> QGSMGSKRQWALEDFEIGRPLGKGKFGNVYLAREKQSKFILALKVLFKAQLEKAGVEHQLRREVEIQSHLRHPNILRLYGYFHDATRVYLILEYAPLGTVYRELQKLSKFDEQRTATYITELANALSYCHSKRVIHRDIKPENLLLGSAGELKIADFGWSVHAPSSRRTTLCGTLDYLPPEMIEGRMHDEKVDLWSLGVLCYEFLVGKPPFEANTYQETYKRISRVEFTFPDFVTEGARDLISRLLKHNPSQRPMLREVLEHPWITANSSKPS

Aurora A is a serine/threonine protein kinase that plays an important role in controlling early stages of mitosis, including centrosome maturation and separation, mitotic entry, and bipolar spindle formation. Localization and enzymatic activity of Aurora A are regulated by its interaction with the spindle assembly factor TPX2. We have used fragment-based, structure-guided lead discovery to develop small molecule inhibitors of the Aurora A-TPX2 protein–protein interaction (PPI). The initial fragment hits identified from screening with the ATP site blocked by a high-affinity inhibitor were very weakly active, but guided by continuous crystallographic analysis of the inhibitors in complex with Aurora A, we were able to increase target affinity by more than 10,000-fold, clearly demonstrating the ability of fragment-based and structural biology approaches to develop potent PPI inhibitors when a suitable binding pocket is present. These compounds occupy a hydrophobic pocket on the surface of Aurora A, discrete from its ATP-binding catalytic site, which forms the interaction surface for a linear N-terminal segment of the interacting peptide from TPX2.

Crucially, we were also able to obtain crystal structures of some of these hits in complex with the Aurora A protein, enabling a structure-based drug design. A representative of such fragment is compound 2, a biphenyl molecule bearing a carboxylic acid and a phenol group on one ring and a lipophilic trifluoromethoxy group on the other. Compound 2 has a KD of 63 μM as measured by our competitive FP assay and a KD of 145 μM as determined by ITC. The binding of 2 to Aurora A, as determined by X-ray crystallography, alongside some key structural motifs showing both the ATP site and TPX2 peptide binding sites, is highlighted in Figure 2. Our ligand-observed Carr-Purcell-Meiboom-Gill (CPMG) NMR experiments and FP studies showed that these fragments are competitive with the TPX2 peptide, and X-ray crystallography revealed that the hit fragments bind to part of the TPX2 binding site, normally occupied by the Tyr8 and Tyr10 of TPX2. An overlay of the crystal structures of early hit 2 with CAM2602 bound to Aurora A reveals a remarkable overlap of the core biaryl scaffold in the two compounds.> GLPTMLTPGSSQFLTSDDFQSPCALPNFDVTPPIHIPGEVFNMMELAEIDSMIPMNSVTGKANTMEMYPIPLDDKGSATPIFSISLSPASDKRLQYTMLGEILNYYTHWTGSLRFTFLFCGSMMATGKILLSYSPPGAKPPTTR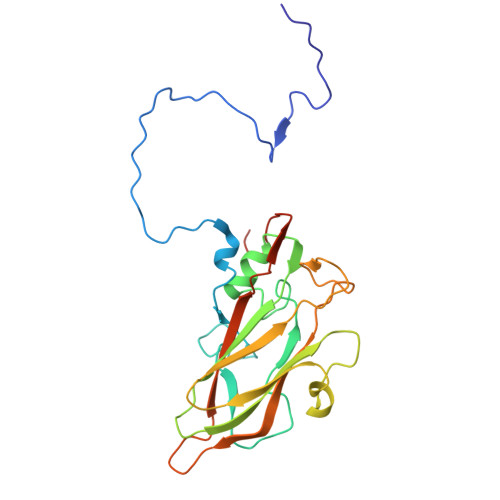KDAMLGTHIIWDLGLQSSCTMLAPWISNTVYRRCIKDDFTEGGYITCFYQTRIVVPSGTPTSMFMLAFVSACPDFSVRLLRDTNHISQRTLFARAQ> GCVRVRTGCRIRCVRASFTYTQAQMYARYRTRSRFYKRPEKMLKAYNVSPNLLRLPKVKPGLLKGIYTDEKIDLRDRERLELVESIRHPKERDFYQDHTYHNQWIARDLESHQKIQIAGRYPYFSPDYEIKPWIWYPGDTVEVVSGEGAGQRGAIIAVVKYKNEILVQNVNVQDVVIPASETRPEQVVQREHPISVLRVRHVDPSTNQLCHLEIVKVRNKETGELEERRISLESGALLPIPAPEETVEAGDPLKDTAIQDADEETYDREKEMPLLVVRRLQAMENYFVDSLQKSHEYHKALQMRNAQDMQTFQKDVLVRATEKLAAAAAVAGHGAMAEAGSQAASVATESSQAGDAEEDAVKGTITVETVVAEVLKSEQRFRSDAAAPGV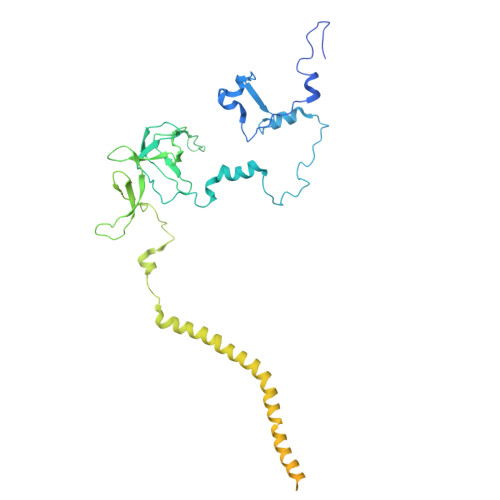PGWWQNMIDAYVSVLEEEEATIEAEAAAQAQAAEADRRAEQLMADATAEAGQSMEEDGTMEGGDEDLDEQDGDLDEDASRSDRSK> MAVLVIKLIPGLSGDIFRAAVELGYRGIVIEGYGAGGIPYRGSDLLQTIEELSKEIPIVMTTQAMYDGVDLTRYKVGRLAL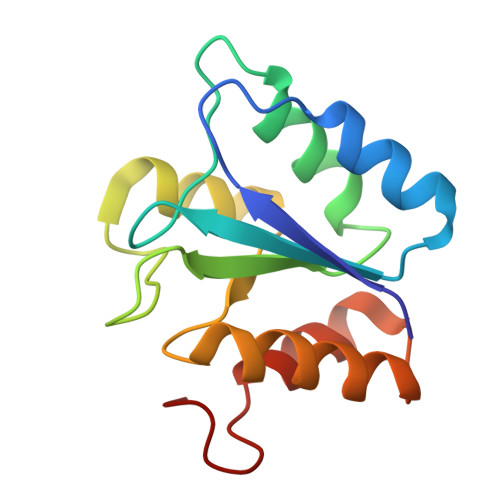RAGVIPAGDMTKEATVTKLMWILGHTNNVEEIKVLMRKNLVGELRD> METREHLFKVLVIGELGVGKTSIIKRYVHQLFSQHYRATIGVDFALKVLNWDSRTLVRLQLWDIAGQERFGNMTRVYYKEAVGAFVVFDISRSSTFEAVLKW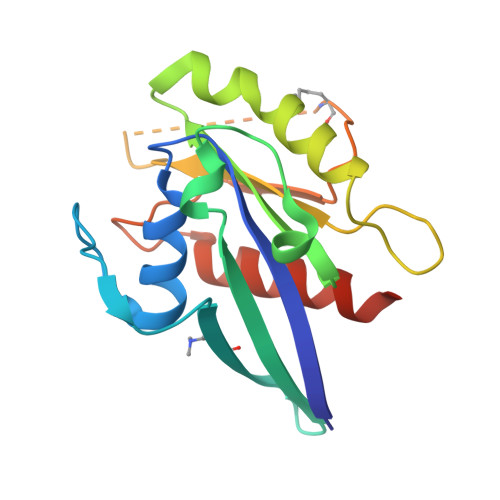KSDLDSKVHLPNGSPIPAVLLANKCDKNKDSSQSPSQVDQFDKEHGFAGWFETSAKDNINIEEAARFLVEKILVNHQSFPN> LPPYDPCAVFNSINYLNLPEVQTALHANVSGIVEYPWTVCSNTIFDQWGQAADDLLPVYRELIQAGLRVWVYSGDTDSVVPVSSTRRSLAA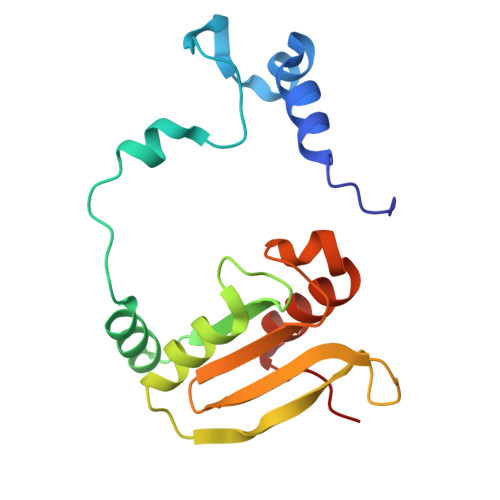LELPVKTSWYPWYMAPTEREVGGWSVQYEGLTYVTVRGAGHLVPVHRPAQAFLLFKQFLKGEPMPAE> IPTPDASMTWNEYDKFYTGSFQETTSYIKFSATVEDCCGTNYNMDERDETFLNEQVNKGSSDILTEDEFEILCSSFEHAIHERQPFLSMDPESILSF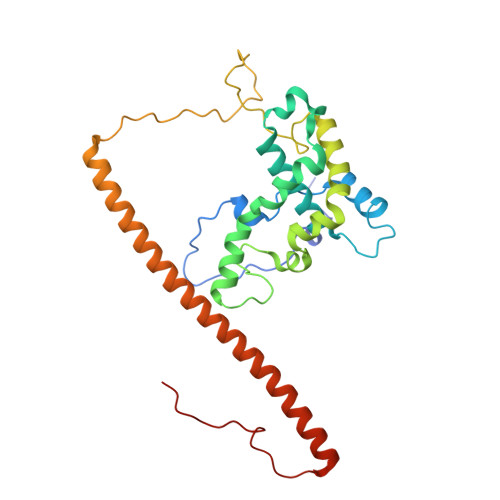EELKPTLIKSDMADFNLRNQLNHEINSHKTHFITQFDPVSQMNTRPLIQLIEKFGSKIYDYWRERKIEVNGYEIFPQLKFERPGEKEEIDPYVCFRRREVRHPRKTRRIDILNSQRLRALHQELKNAKDLALLVAKRENVSLNWINDELKIFDQRVKIKNLKRSLNISGEDDDLINHKRKRPT>[4x]GSNNQLVVRAKFNFQQTNEDELSFSKGDVIHVTRV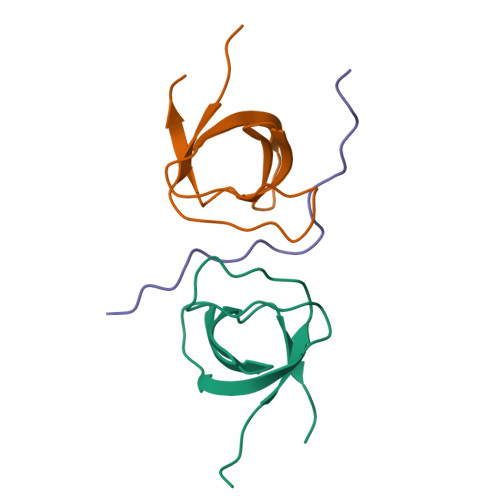EEGGWWEGTLNGRTGWFPSNYVREVKA;>GSGGGKPSRPPRPSRPPPPTPRRPASY[2x]>[4x]MKFSNITIKNFRNFEKVNINLDNKNVIFGMNDIGKTNFLYALRFLLDKEIRKFGFNKSDYHKHDTSKKIEIILTLDLSNYEKDEDTKKLISVVKGARTSANADVFYIALESKYDDKELYGNIILKWGSELDNLIDIPGRGNINALDNVFKVIYINPLVDLDKLFAQNKKYIFEESQGNESDEGILNNIKSLTDQVNQQIGEMTIIKGFQQEITSEYRSLKKEEVSIELKSEMA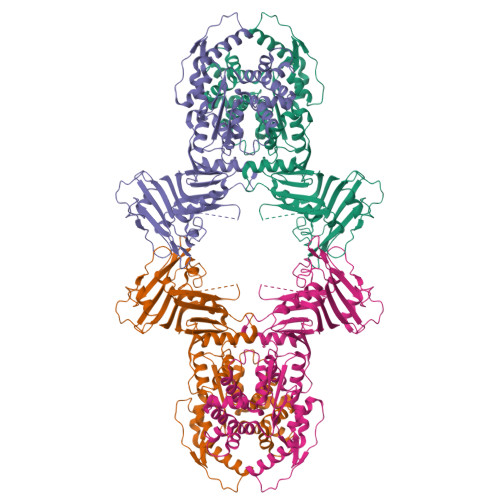IKGFFSDIIPYIKKDGDSNYYPTSGDGRRKMLSYSIYNYLAKKKYEDKIVIYLIEEPEISLHRSMQIALSKQLFEQSTYKYFFLSTHSPELLYEMDNTRLIRVHSTEKVVCSSHMYNVEEAYGSVKKKLNKALSSALFAERVLLIEGPSEKILFEKVLDEVEPEYELNGGFLLEVGGTYFNHYVCTLNDLGITHIIKTDNDLKSKKGKKGVYELLGLNRCLNLLGRENLDEITIDIPEDIKGKKKKERLNERKKEIFKQYKNEVGEFLGERIYLSEIDLENDLYSAIGESMKRIFENEDPVHYLQKSKLFNMVELVNNLSTKDCFDVFEHEKFACLKELVGSDRG>[2x]MKKTKIVCTIGPKTESEEMLAKMLDAGMNVMRLNFSHGDYAEHGQRIQNLRNVMSKTGKTAAILLDTKGTEIRTMKLEGGNDVSLKAGQTFTFTTDKSVIGNSEMVAVTYEGFTTDLSVGNTVLVDDGLIGMEVTAIEGNKVICKVLNNGDLGENKGVNLPGVSIALPALAEKDKQDLIF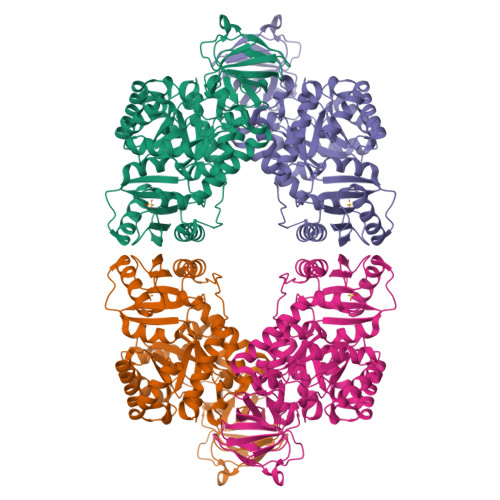GCEQGVDFVAASFIRKRSDVIEIREHLKAHGGENIHIISKIENQEGLNNFDEILEASDGIMVARGDLGVEIPVEEVIFAQKMMIEKCIRARKVVITATQMLDSMIKNPRPTRAEAGDVANAILDGTDAVMLSGESAKGKYPLEAVSIMATICERTDRVMNSRLEFNNDNRKLRITEAVCRGAVETAEKLDAPLIVVATQGGKSARAVRKYFPDATILALTTNEKTAHQLVLSKGVVPQLVKEITSTDDFYRLGKELALQSGLAHKGDVVVMVSGALVPSGTTNTASVHVL> GAMKIAFIGEAVSGFGGMETVISNVIHTFENSSPKINCEMFFFCRNDKMDKAWLKEIKYAQSFSNIKLSFLRRAKHVYNFSQWLKETSPDIVICIDVISCLYANKARKKSGKHFTIFSWPHFSLDHKKHAECITYADYHLAISSGIKEQIMARGISAQDISVVYNPVSIKTVIVPPPERDKPAVFLYVGRLKFEGQKRVKDLFDGLARTTGEWQLHIIGDGSDFEKCQAYSRELGIEQRVIWYGWQSAPWQVVQQKIKN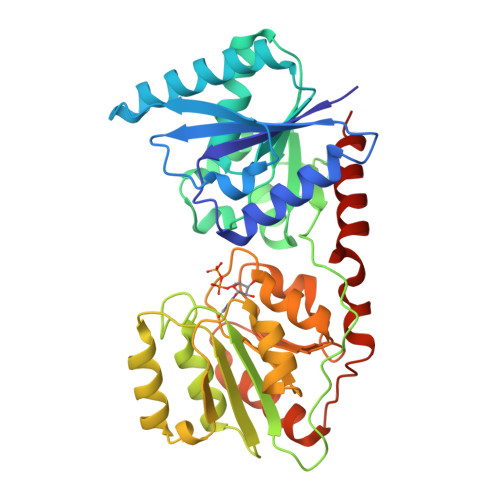VTALLLTSAFEGFPMTLLEAMSYGIPCISSDCMSGPRDMIKPGLNGELYTPGAIDDFVGHLNRVISGEVKYQHDIIPGTIERFYDVLYFKNFNNAIFSKLQK> GPGSSRWSKDYDVCVCHSEEDLVAAQDLVSYLEGSTASLRCFLQLRDATPGGAIVSELCQALSSSHCRVLLITPGFLQDPWCKYQMLQALTEAPGAEGCTIPLLLGLSRAAYPPELRFMYYVDGRGPDGGFRQVKEAVMR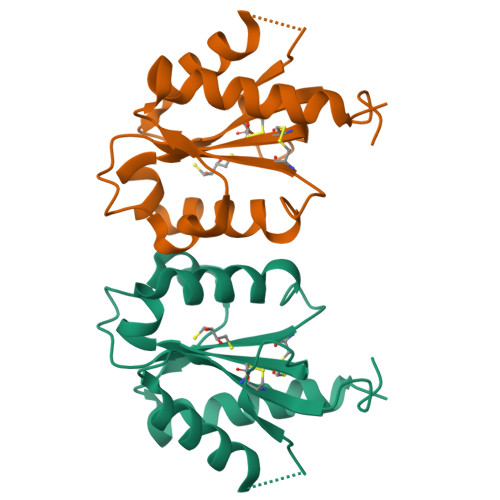YLQTLS>[2x]GPGMSASGSGDATLGIVHTLMCHRQGGESENFAKRAVESLVKKLKDKRDELDALITAVTSNGIQQSKCVTIARTL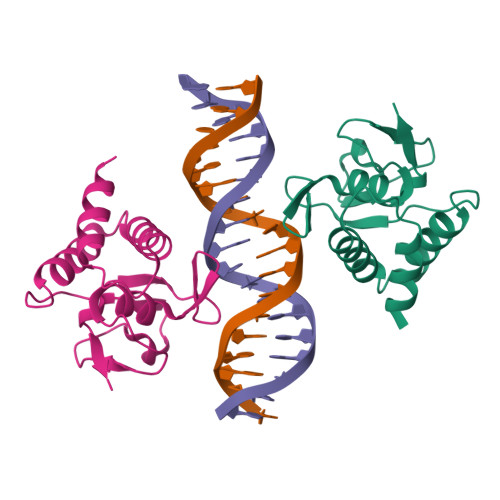DGRLQVAGKKGFPHVIYSRIWRWPDLHKNELKHIKLCKFAFDLKLDHVCVNPYHYERVISPGYNVTDI> AMPSYNNARLLEKRLQNCDTQLNQFFNGQELSIKFLQQLNQI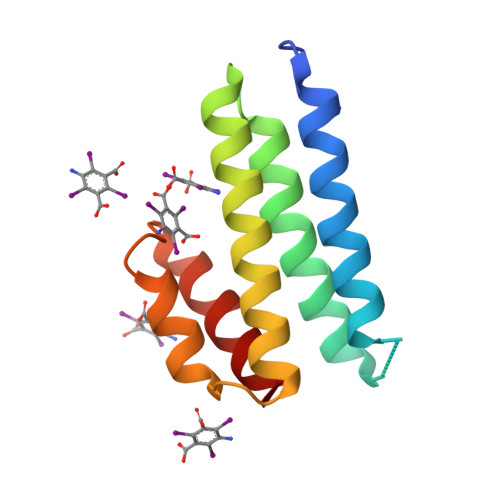KYFYNSAFNKTENEDDGLEVVEEYENFISLVSQVKSGQINADKAFETIKDTTESRQADVIIANFFKVCE>[2x]GPLGSRQWALEDFEIGRPLGKGKFGNVYLAREKQSKFILALKVLFKAQLEK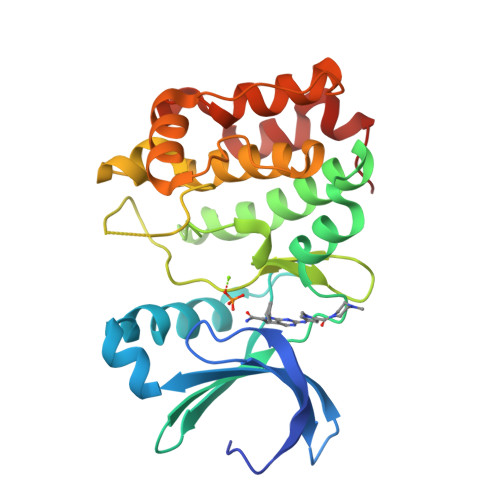AGVEHQLRREVEIQSHLRHPNILRLYGYFHDATRVYLILEYAPLGTVYRELQKLSKFDEQRTATYITELANALSYCHSKRVIHRDIKPENLLLGSAGELKIADFGWSVHAPSSRRDDLCGTLDYLPPEMIEGRMHDEKVDLWSLGVLCYEFLVGKPPFEANTYQETYKRISRVEFTFPDFVTEGARDLISRLLKHNPSQRPMLREVLEHPWITANSSKPS> GSTLQPLENSTRQEKLLYPKLNQLSNSINAAVAFLLEARNLEGWWQDFNFPQAASIGDEWVTAYVGTMLATLPYAHVHEALMQAWELLKIRDHRPTGEWGYNYILCGDANTTGWAL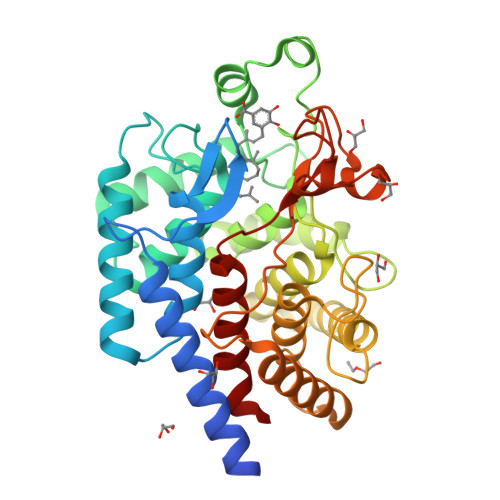QLAAAVGASDSERAQQARAALATHLQPNGGIATFAEESIRAYIKVPDLANVSFQGWCGAHTCVSAAVAALPEFRSRLHDYLRVTQTSQGNWEGYWWSDHEYTTALTAEALAAGGQAADQPSIEQAVAWGLKRLCPQGFVATSKHPNGSTFATAWCLRLLLLNTVDAEVKAARAAAIGWLLEQQRPNGSWVSSAYLRIPYPFDRNPNQFPHWRYYDEIEGDKRFEGSIIFDHNSIFTTATVVNSLVKAAPML>CG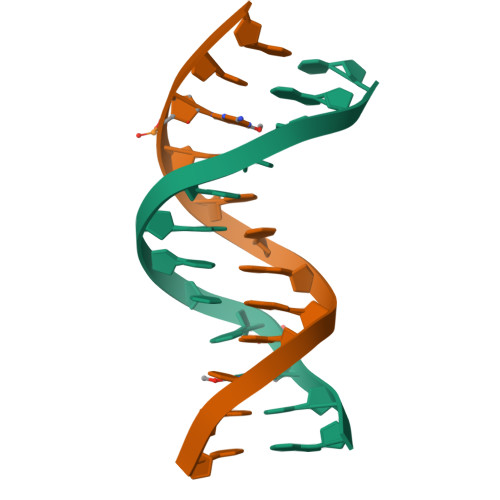TGAATTCGCG[2x]> MPTQKELRDTMSKKLQEAIKHPDPAVVAGRKSAIKRWVGVLQDNFMEHIKYFKGDKLKFLHNVFQDEGCWSGVRLDNAALGQRFTEEKIGGIDNPLRKYEMACSYCVVDKIHPLFQKRFESYRNKFPPGAFDGKTETEFGKYVRNSLLDSIKRKGPVFDFWIDRESGELKKYDAVEGFDSAVKFKWSEGVEYFYNHLKEEDKEKKLTEAILALSRVQSVEKDAPILDFCVNKIVDKDTLLQKLSQKDKGVYSLFAELIESCFFDTVHDLVQCWCYKEVSAGGDHSEKIFSQRDYELFLSSLSDTMLKNPELSVQARSLIMEFWECGSLYQYRKAAVNTSNYTVPTSGVFAELIVNWRREDIYKTDEEKEIEKKEILDMMSFAKDCFPEKFELFKKLIIRDLRLCGREGKRVNVDYGLFAEELFSELEKTILPPGPVGDGPCSNLRSRSKAHGSKKTTLPVDDSPQSELGTPSVSGVSSYKKKSVFTLSGNKLEHHHHHH;> MSNGDGLIRSLVDGDLEGFRQGFESFLDQCPSFLYHVSAGRFLPVFFFSMFSTAHDANILNANERVYFRFDNHGVNPRNGENRNTANLKVAVYRDGQQVVRCYSISDRPNSDGLRFSTRERNALVQEIRRQNPNLREEDLNFEQYKVCMHGKGKSQGEAIATVFEVIREKDRQGRDKFAKYSASEVHFLRQLFRNHRLTIKEIEGRQLNQNQLRQLGRSVNFTRVEPGQQRIDNFMEMLASNQRQDVRDSLRGDILEYVTDTYNNYRAQIENNIEGRSQKFESHGFLLGFLANFSHRYTIGVDLDLSPRNSHVAFLVRHQVERENIPIVINLATRAPPYIALNRARSHAERLHVFSFIPIHTESRNTVCVGLNFNLNLDPFSVDTVGLQQDRFPLVQRLFECLENEGIRENIRDFLLHHLPAEIPRNAENYDRIFDCITGFAFGNSAFDRHPLELEEEDEAPITKYIFRHGDEGLRCLTMVFHAEGSDIVILHIRAHDAQQQGAINLQTLNVNGNDVHVWEVSCTLNNQLELDIDLPNDLGLYHDYQNNNANNFLAGDLVQVPNTENVHNTLNQVVNDGWKNIAQHRGLFQEISGALMPLVDTINVNSEDKFRSILHGTFYASDNPYKVLAMYKVGQTYSLKRGQEEEGERV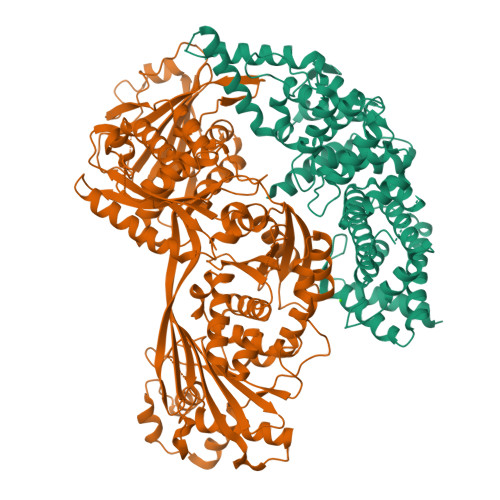ILTRITEQRLDLLLLRQPRENDLDTHPIGYVLRLANNAEEVGQQQNDARQEIGRLKKQHRGFIPITSGNEVVLFPIVFNRDAHEAGNLILFPEGIGREEHVHRLDRHVRLEHHHHHH> KPACYACK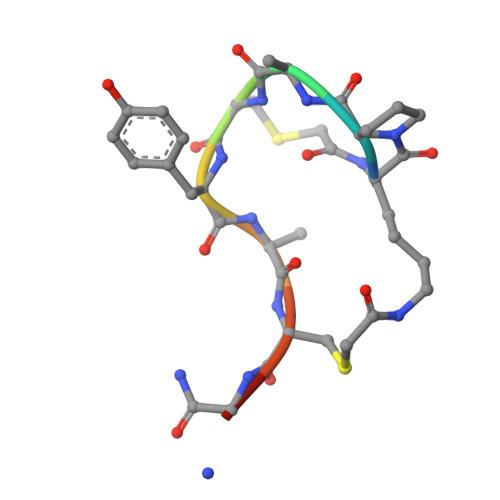A> MPVITVNTNVAEKSIPVFFQAALTNMMTKALQKPKEVMFVDLRSGANIMMGGDRNPCVFATVECIGRLNP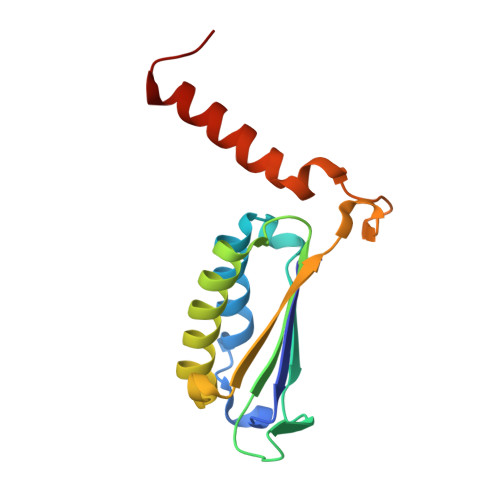TSNLAMARDMEDMFIEHLNVRRERIVIRFIPVPALFCSFNGALHDVSIERDEDIISQAIAEYLHHHHHHH> NVHSNYTFIIAGGGISGLTLADRLTEDPRVTVLVIEAGPLDRGEDGILVPGAFSPWLYFWPGLVSTPQAGLNNRTVDVITAQVVGGGSTINAMVYLRGDKDDYDSWGALGNPGWSWNSMLPYFIKSETFTPPSPELAAAGNITWDGSIRGRSGPVNYSYPNYFFPGSENWWNAANEVGLPPVKDPMAGSKQGVFWIPSAIDARTMTRSHARRNHYDRVSSRPNYHILPSHLVSKILFRGKQAIGVSYIPTSGGNTTTNVYASKEITLAAGGLGTPKILQLSGIGPRKLLNELGIPVISDLPGVGQNLQDQPTLTIPYTFTNNVFPNTDSLTTNATYNAEQRALYDSSKQGAYTIVNSLSTNIGVMSLQRAAPKSYRQIIAAARARSASLSLPPGTDPAVIRGYQAQRNAILKQFENPNVGVGTVHWGTGSSALVYHLKPLSRGTVNIRSTNPLDAPEIDYRTGTDPIDAQVYTSLFRKNREIFNAPSMRVLGPSEAAPFGANLTTDEEIYAVMRELINPSNAHQCCTAAMMPKDMGGVVSSEQKVYGVQGLRVADISFWPFQLSGSPMATAYAGAERLADVIKKEHRLAGAPKSL

The FAD-dependent oxidoreductase from Chaetomium thermophilum (CtFDO) is a novel thermostable glycoprotein from the glucose–methanol–choline (GMC) oxidoreductase superfamily. However, CtFDO shows no activity toward the typical substrates of the family and high-throughput screening with around 1000 compounds did not yield any strongly reacting substrate. The structure of CtFDO reveals an unusually wide-open solvent-accessible active-site pocket with a unique His–Ser amino-acid pair putatively involved in enzyme catalysis. A series of six crystal structures of CtFDO complexes revealed five different subsites for the binding of aryl moieties inside the active-site pocket and conformational flexibility of the interacting amino acids when adapting to a particular ligand.

Despite marginal differences in the crystallization conditions used for the preparation of the complexes, polymorphism can be observed, as demonstrated by three different space groups: P212121 for CtFDO:PESB, CtFDO:4NC, CtFDO:4NP and CtFDO:ABTS, P21212 for CtFDO:MAMB and P21 for CtFDO:IPEA and CtFDO:free. The position of the active-site water WAS (HOHA836) is similar to that in CtFDO:free (shifted by 0.7 Å). MAMB is hydrogen-bonded to Tyr476 and, via WAS, to flavin. One additional water mediates the contact of MAMB with Asn562. MAMB is further stabilized by van der Waals (vdW) interactions with the flavin, Ala133, Leu399, Tyr476 and Asn562. The formic acid molecule interacts via hydrogen bonds to Thr464, Ser607 in both conformers and, via a water molecule, to Gln351.>[6x]MDEQEFRKQLTLKPVEEEHIDQFNELLSYVFQVTEADIEESGFENKRAFIKSKQPILELSKVFGWFHENQLISQIAIYPCEVNIHGALYKMGGVTGVGTYPEYANHGLMKDLIQTALEEMRQDKQWISYLFPYNIPYYRRKGWEIMSDKLSFKIRDTQLPKTVPVPGMIERLAVDHPDVFDVYARFARQNHGALIRSAFNWEEYWRFENEEERTAAVYYGANQE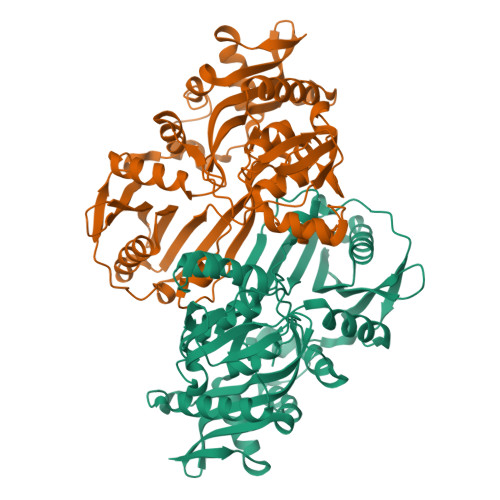PLGVLFYWVADEVFHIKEMFYLNQEARNGLWNFITAHFSMVYWVKGDIYKNEPLAFLLEDSQIKESIEPYYMARIVDVKAFLENFPFESTAKPFHFVVKDPVAEWNNGIFGLIWDENDQVTITDEPLGTAVHLDIQTLTCLVMNYRRPSYLHRIERIDTDKETLNSLERIFPDQEAYFSDYF>MMEQVCDVFDIYAICACCKVESKNEGKKNEVFNNYTFRGLGNKGVLPWKCNSLDMKYFCAVTTYVNESKYEKLKYKRCKYLNKETVDNVNDMPNSKKLQNVVVMGRTSWESIPKKFKPLSNRINVILSRTLKKEDFDEDVYIINKVEDLIVLLGKLNYYKCFIIGGSVVYQEFLEKKLIKKIYFTRINSTYECDVFFPEINENEYQIISVSDVYTSNNTTLDFIIYKKTNNKMLNEQNCIKGEEKNNDMPLKNDDKDTCHMKKLTEFYKNVDKYKINYENDDDDEEEDDFVYFNFNKEKEEKNKNSIHPNDFQIYNSLKYKYHPEYQYLNIIYDIMMNGNKQSDRTGVGVLSKFGYIMKFDLSQYFPLLTTKKLFLRGIIEELLWFIRGETNGNTLLNKNVRIWEANGTREFLDNRKLFHREVNDLGPIYGFQWRHFGAEYTNMYDNYENKGVDQLKNIINLIKNDPTSRRILLCAWNVKDLDQMALPPCHILCQFYVFDGKLSCIMYQRSCDLGLGVPFNIASYSIFTHMIAQVCNLQPAQFIHVLGNAHVYNNHIDSLKIQLNRIP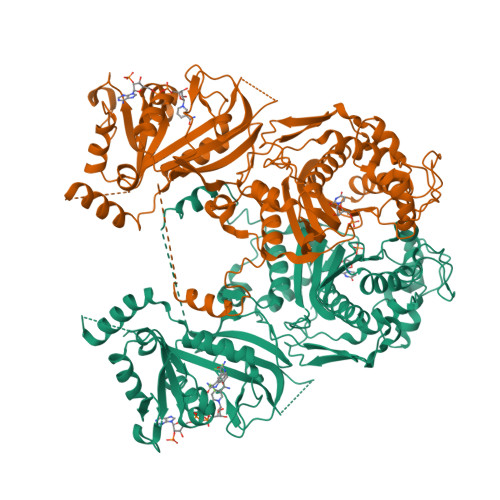YPFPTLKLNPDIKNIEDFTISDFTIQNYVHHEKISMDMAA[2x]> MTTVAPERLSRIREIIAENIDVDLDGLSDTALFIDELGADSL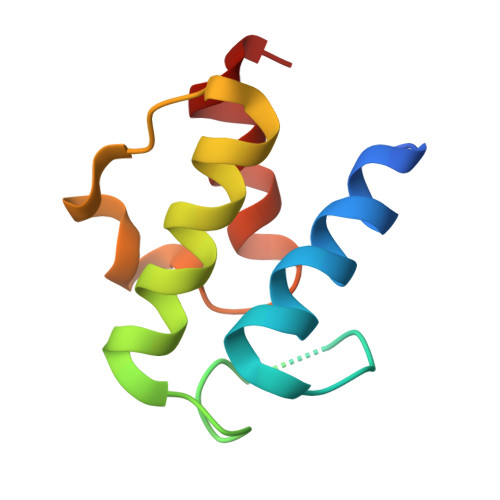KLIDVLSALEMEYSIVIDMNELPKMTNVEATYQVTAAAAGW>MGFVVALIQGDGIGPEVVSKSKTILARLNEKFSLPIEYIEVEAGDTTKNKFGDALPKDSLRVIEKADMILKGPVGETAADVVVKLRLMYDLYANLRPAKSLPGLENKFGDVDILVVRENTEDLYKGLEHVISDGVTVGIKVITRAASTRIAQVALNQALRRKKKVVCVHKSNVMRITDGLFAESCRNVLKGKVEYSEMYVDAAAANLVRNPQAFDVIVTENTYGDILSDEAGQIAGSLGISPSANIGDRKSLFEPVHGAAFD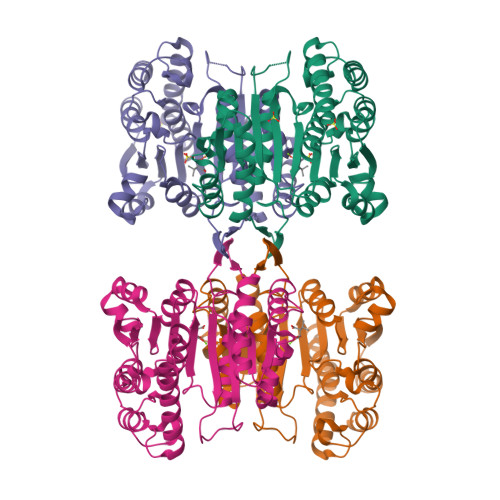IAGKNIANPTAFLLSVGMMLDRMQELSGDIRYNNAAKSLRDAIYSVYSEGKYLTPDVGGSSTTDEMISAIRSKIG[2x]>SMKHPLEELKDPTENLLLWIGRFLRYKCTSLSNSQVKDQNKVFECLNELNQACSSSQLEKVCKKARNAGLLGINTYALPLLKFHEYFSKARLITERLAFNSLKNIDEVMLAEFLSVYTGGLSLATKKNYRIALLGLFSYIDKQNQDENEKSYIYNITLKNISGVNQSAGNKLPTHLNNEELEKFLESIDKIEMSAKVRARNRLLIKIIVFTGMRSNEALQLKIKDFTLENGCYTILIKGKGDKYRAVMLKAFHIESLLKEWLIERELYP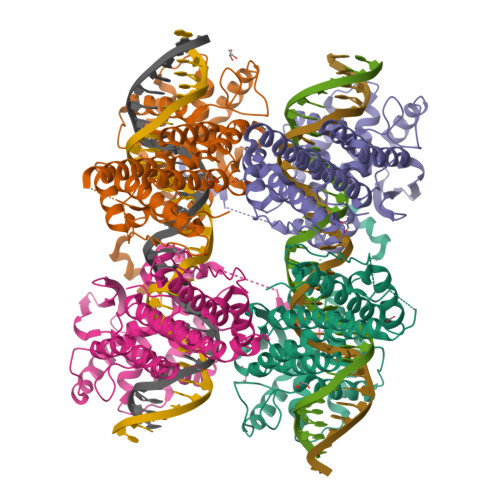VKNDLLFCNQKGSALTQAYLYKQVERIINFAGLRREKNGAHMLRHSFATLLYQKRHDLILVQEALGHASLNTSRIYTHFDKQRLEEAASIWEEN[4x]Rab GTPases play a crucial role in vesicular trafficking through shuttling between cytosol and membranes, a process that is controlled by several regulatory proteins. Another translocated effector protein LidA is also involved in the recruitment of early secretory vesicles to the LCV. LidA was found to interact with Rab1 as well, regardless of nucleotide binding states, and promote SidM/DrrA activity of transporting Rab1 to the LCV. Here, we present the crystal structures of LidA (residues 224-559) in complex with a GDP-bound Rab1 mutant (S25N; residues 1-176) and LidA (residues 188-449) in complex with GTP-bound Rab1 (residues 1-176).

To reveal the molecular basis for the LidA-Rab1 interaction, we first solved the crystal structure of LidA(224-559) in complex with a constitutively GDP-bound mutant Rab1(S25N; 1-176) at 1.73 Å using molecular replacement. The overall LidA-Rab1 complex adopts a compact and globular structure. The interaction between LidA and Rab1 resulted in a 1∶1 stoichiometric complex and buried 41% (4031 Å2/9845 Å2) of the Rab1. In the structure, Rab1 is held in a large and pronounced groove made by the four “fingers” with an extensive, though not complete, charge and surface complementarities. Contacts between LidA and Rab1 are established through a combination of hydrogen bonds and hydrophobic interactions involving the switch I, switch II and the interswitch region of Rab1. LidA (residues 224-559) is composed of seven α-helices and ten β-strands, which arrange into a structure resembling a hand with the baby finger buried in the palm and the remaining four straightened. Unexpectedly, the structures showed that GDP-Rab1(S25N), a “constitutively” inactive mutant, adopted an active conformation when bound by LidA. Surprisingly, structural comparison revealed that the conformation of LidA-bound Rab1(S25N) is essentially identical with that of LidA-bound GTP-Rab1, indicating that Rab1(S25N) is in the active conformation following LidA binding. As with GTP, LidA binding induces striking structural remodeling around the switch I region of Rab1(S25N), which swings from the edge of β-sheet to the nucleotide-binding site, with the largest displacement of 9.2 Å at the Cα atom of Ile. Despite loss of the γ phosphate group-mediated interactions, the switch I region in Rab1(S25N) is stabilized through its interaction with α7 of LidA.

> GPLGSMSSMNPEYDYLFKLLLIGDSGVGKNCLLLRFADDTYTESYISTIGVDFKIRTIELDGKTIKLQIWDTAGQERFRTITSSYYRGAHGIIVVYDVTDQESFNNVKQWLQEIDRYASENVNKLLVGNKCDLTTKKVVDYTTAKEFADSLGIPFLETSAKNATNVEQSFMTMAAEIKKRM;> KKLDKLERQGKDLEDKYKTYEENLEGFEKLLTDSEELSLSEINEKMKAFSKDSEKLTQLMEKHKGDEKTVQSLQREHHDIKAKLANLQVLHDAHTGKKSYVNEKGNPVSSLKDAHLAINKDQEVVEHKGQFYLLQKGQWDAIKNDPAALEKAQKDYSQSKHDLATIKMEALIHKLSLEMEKQLETINDLIMSTDPKENEEATKLLHKHNGLNLKLANLQDMLAVHRKEKSFFNEKGEKVTSLNDAHYVIGKDQQLFNLGGKFYPIHKEQKILEKDGKFYLLKQGEDWESIKDSPEKQKKAEHDFHKLQYETPMTVKKLVHHNKGLETTIHKERIEELEHHHHHH> MDVKQVEKKDSVDKTNAEENKDSSVKPAENATKAELKGQVKDIVEESGVDTSKLTNDQINELNKINFSKEAKSGTQLTYNDFKKIAKTLIEQDARYAIPFFNASKIKNMPAAKTLDAQSGKVEDLEIWDSWPVQDAKTGYVSNWNGYQLVIGMMGVPNVNDNHIYLLYNKYGDNDFNHWKNAGPIFGLGTPVIQQWSGSATLNKDGSIQLYYTKVDTSDNNTNHQKLASATVYL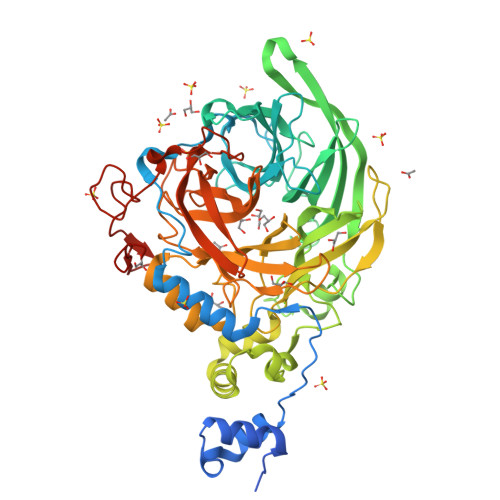NLEKDQDKISIAHVDNDHIVFEGDGYHYQTYDQWKETNKGADNIAMRDAHVIDDDNGNRYLVFEASTGTENYQGDDQIYQWLNYGGTNKDNLGDFFQILSNSDIKDRAKWSNAAIGIIKLNDDVKNPSVAKVYSPLISAPMVSDEIERPDVVKLGNKYYLFAATRLNRGSNDDAWMATNKAVGDNVAMIGYVSDNLTHGYVPLNESGVVLTASVPANWRTATYSYYAVPVEGRDDQLLITSYITNRGEVAGKGMHATWAPSFLLQINPDNTTTVLAKMTNQGDWIWDDSSENPDMMGVLEKDAPNSAALPGEWGKPVDWDLIGGYNLKPHQHHHHHH>SDELYRQSLEIISRYLREQATGAKDTKPMGRSGATSRKALETLRRVGDGVQRNHETAFQGMLR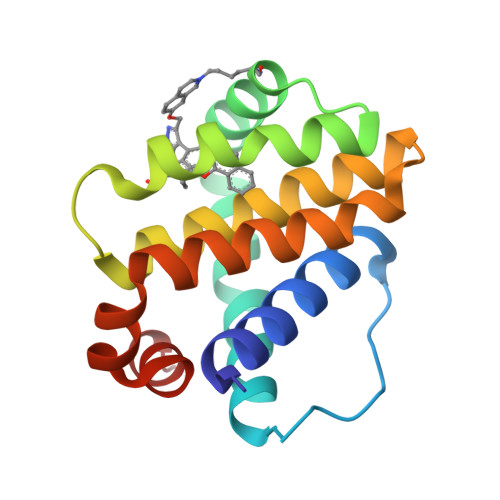KLDIKNEDDVKSLSRVMIHVFSDGVTNWGRIVTLISFGAFVAKHLKTINQESCIEPLAESITDVLVRTKRDWLVKQRGWDGFVEFFHVE[2x]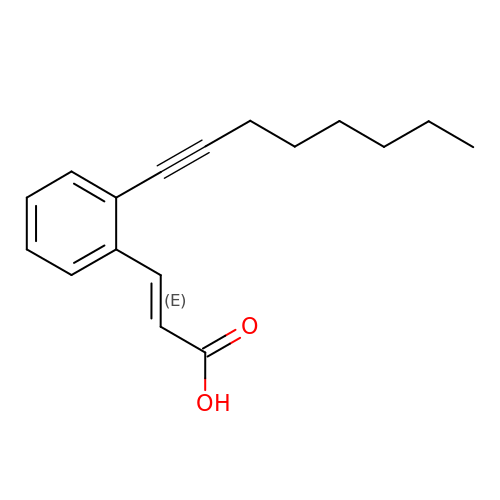(2E)-3-(2-OCT-1-YN-1-YLPHENYL)ACRYLIC ACID | C17 H20 O2 | KRDSGPLHVQJFLM-BUHFOSPRSA-N> IGDEPLENYLDTEYFGTIGIGTPAQDFTVIFDTGSSNLWVPSVYCSSLACSDHNQFNPDDSSTFEATSQELSITYGTGSMTGILGYDTVQVGGISDTNQIFGLSETEPGSFLYYAPFDGILGLAYPSISASGATPVFDNLWDQGLVSQDLFS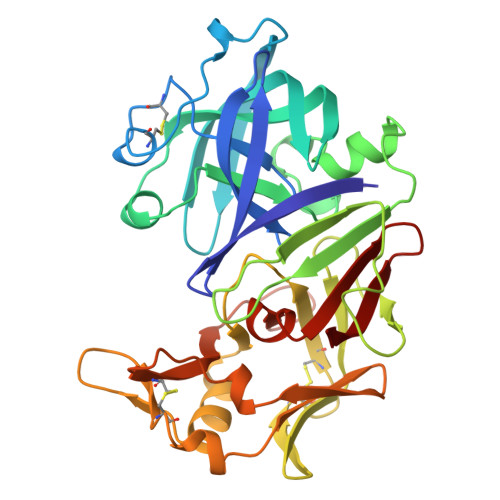VYLSSNDDSGSVVLLGGIDSSYYTGSLNWVPVSVEGYWQITLDSITMDGETIACSGGCQAIVDTGTSLLTGPTSAIANIQSDIGASENSDGEMVISCSSIASLPDIVFTINGVQYPLSPSAYILQDDDSCTSGFEGMDVPTSSGELWILGDVFIRQYYTVFDRANNKVGLAPVA> GHMDQETIDTDYDVIVLGTGITECILSGLLSVDGKKVLHIDKQDHYGGEAASVTLSQLYEKFKQNPISKEERESKFGKDRDWNVDLIPKFLMANGELTNILIHTDVTRYVDFKQVSGSYVFKQGKIYKVPANEIEAISSPLMGIFEKRRMKKFLEWISSYKEDDLSTHQGLDLDKNTMDEVYYKFGLGNSTKEFIGHAMALWTNDDYLQQPARPSFERILLYCQSVARYGKSPYLYPMYGLGELPQGFARLSAIYGGTYMLDTPIDEVLYKKDTGKFEGVKTKLGTFKAPLVIADPTYFPEKCKSTGQRVIRAICILNHPVPNTSNADSLQIIIPQSQLGRKSDIYVAIVSDAHNVCSKGHYLAIISTIIETDKPHIELEPAFKLLGPIEEKFMGIAELFEPREDGSKDNIYLSRSYDASSHFESMTDDVKDIYFRVTGHPLVLKQRQEQEKQ;> MNSEYDYLFKLLLIGNSGVGKSCLLLRFSDDTYTNDYISTIGVDFKIKTVELDGKTVKLQIWDTAGQERFRTITSSYYRGSHGIIIVYDVTDQES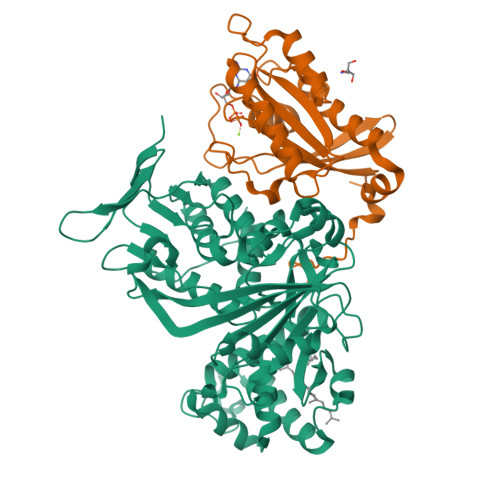FNGVKMWLQEIDRYATSTVLKLLVGNKCDLKDKRVVEYDVAKEFADANKMPFLETSALDSTNVEDAFLTMARQIKESMSQQNLNETTQKKEDKGNVNLKGQSLTNTGGCCC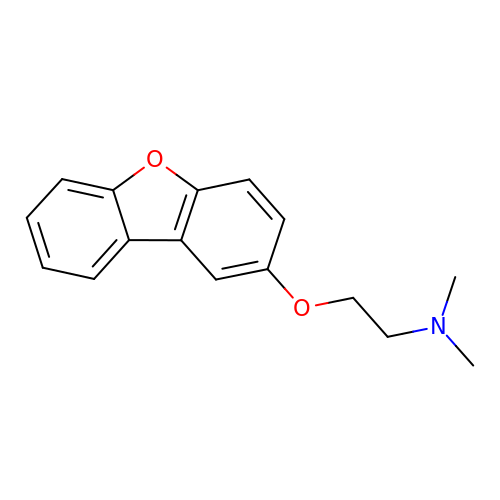2-[(dibenzo[b,d]furan-2-yl)oxy]-N,N-dimethylethan-1-amine | C16 H17 N O2 | GQEGJXFTHBKSKR-UHFFFAOYSA-N> VSLELPFETRTWRLQNGLVVTLMPRPALHQTYAMFATRYGSVDRAFRTDGQVHEMPDGIAHFLEHKMFEDPEMDVFARFAAHGASVDAYTTFDHTAYYFSGTGEIAKHVGTLLDFVQSIHLTDENVEKEKGIIAQEIHMVNDHPDRRAYMELLRAMYHEHPVRIDIAGTVESVRAITKEQLLLCYDTFYHPSNMVLVIAGGFDADEIAHVIEENQAKKSFKEPPAIERLYPEEPPTPARSRHWMHFPVQQPRLLVGWKEANGAFGSNLIEQDTAMTI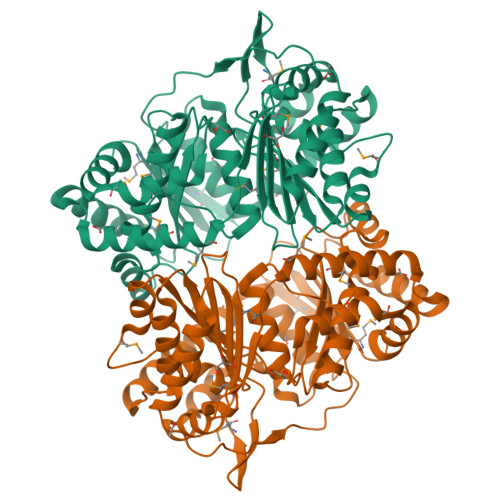LLDALFGPTSAFYQSLLDEGLVDKGFSANYQLSNTFGYTLVGGNAPHPDVLAERIQSHLARVRERGIDEEAFERARKKIMGRVLMSLDQNAFLVRNWVTYFLRGAEAFAFADVIAVLQTMTLERANARFQEHLREDNMVVSAVLPS Sorcin (Soluble resistance-related calcium binding protein) is a calcium binding oncoprotein expressed at high levels in several human tumours, such as leukaemia, gastric, breast and ovarian cancers. Each monomer of Sorcin homodimer is formed by two domains, i.e. a flexible, glycine-rich N-terminal domain and a C-terminal calcium-binding domain (SCBD), endowed with five EF-hands3031. The SCBD can be divided in two regions: EF1–3 (residues 33–134), which binds calcium with high affinity, and EF4–5 (residues 135–198), which mediates dimerization. Upon calcium binding Sorcin undergoes a large conformational change that allows it to bind and regulate a series of target proteins in a calcium-dependent fashion.

In CaSor, Ca2+ is bound at EF1, EF2 and EF3 and it is hepta-coordinated in a classical pentagonal bipyramidal configuration. EF1 and EF2 are coupled by Gln48, which coordinates the EF1-bound Ca2+, whereas in EF2 is hydrogen-bound to Thr89. The binding of calcium to Sorcin promotes a large conformational change, which involves a tilt of the D-helix with respect to the G-helix, with EF3 acting as a hinge. The opening of EF1 and EF3 causes the exposure of two distinct hydrophobic surfaces that likely mediate the interaction of Sorcin with its molecular partners. The analysis of the CaSor structure reveals the presence of an electron density peak in the cavity formed upon calcium binding and the consequent tilt of the D-helix. We fitted this electronic density map with the GYYPGG hexapeptide belonging to the N-terminal region of Sorcin (residues 12–17). We can exclude PEG binding to Sorcin structure: the Fo-Fc and 2Fo-Fc electron density maps shows clearly the presence of a short peptide containing side chains with a very well resolved proline residue clearly visible in the structure (12-GYYPGG-17), belonging to a different dimer. The residues buried at the interface between peptide and Sorcin are: Met78, Met81, Leu82, Glu97, Ala100, Val101, Gly104, Trp105, His108 placed on the D helix; Phe112 on the EF3 loop; Thr131, Met132, on the EF4 loop; Val164, Arg167, and Asp171 on the G helix. Trp105, Glu97 and Arg167 form hydrogen bonds with Tyr13 and Tyr14 of the peptide (OH Tyr13-OE2 Glu97 = 2.78 Å; O Tyr13-NE1 Trp35 = 2.74 Å; O Tyr14-OE2 Glu97 = 2.90 Å). The residues laying on the D helix play a major role in interacting with the N-terminal peptide; in particular, Trp105 establishes a strong stacking interaction with Pro15 and is hydrogen bonded to the carbonyl group of Tyr13, determining the orientation of the peptide into the pocket which is opposite to that of Alix in PDCD6 (see below).

> MAYPGHPGAGGGYYPGGYGGAPGGPAFPGQTQDPLYGYFAAVAGQDGQIDADELQRCLTQSGIAGGYKPFNLETCRLMVSMLDRDMSGTMGFNEFKELWAVLNGWRQHFISFDTDRSGTVDPQELQKALTTMGFRLSPQAVNSIAKRYSTNGKITFDDYIACCVKLRALTDSFRRRDTAQQGVVNFPYDDFIQCVMSV;> MAYPGHPGAGGGYYPGGYGGAPGGPAFPGQTQ>GHMSGSLARAAARPNAPTLVDEATVDDFIAHSGKIVVLFFRGDAVRFPEAADLAVVLPELINAFPGRLVAAEVAAEAERG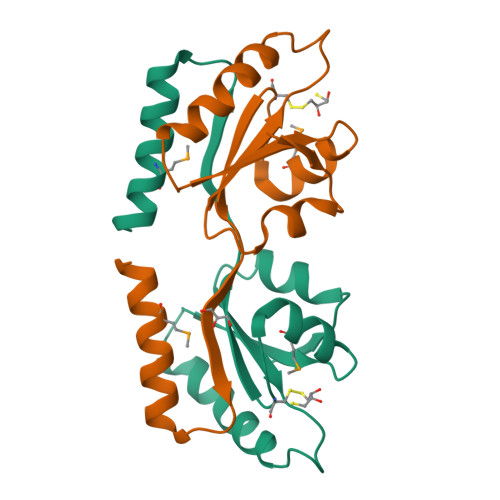LMARFGVAVCPSLAVVQPERTLGVIAKIQDWSSYLAQIGAMLAEVDQPGEAELQSGS[2x]>[4x]AECSVDIAGNDGMQFDKKEITVSKSCKQFTVNLKHPGKLAKNVMGHNW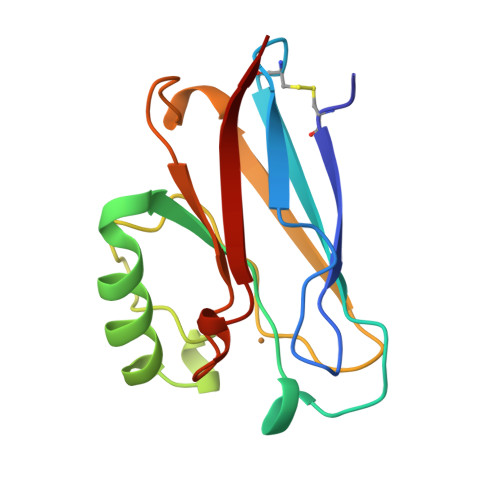VLTKQADMQGAVNDGMAAGLDNNYVKKDDARVIAHTKVIGGGETDSVTFDVSKLAAGEDYAYFCSFPGHFALMKGVLKLVD> GLGDLIEGVVEGVTRNALTPLTPANNLPDTQSSGPAHSKETPALTAVETGATNPLVPSDTVQTRHVIQKRTRSESTVESFFARGACVAIIEVDNDAPTKRASKLFSIWKITYKDTVQLRRKLEFFTYSRFDMELTFVVTSNYTDANNGHALNQVYQIMYIPPGAPIPGKWNDYTWQTSSNPSLFYTYGAPPARISVPYVGIANAYSHFYDGFAKVPLAGQASTEGDSLYGAASLNDFGSLAVRVVNDHNPTKLTSKIRVYMKPKHVRVWCPRPPRAVPYYGPGVDYKDGLAPLPEKGLTTY;> MGAQVSSQKVGAHENSNRAYGGSTINYTTINYYRDSASNAASKQDFAQDPSKFTEPVKDVLIKTAPTLNSPNIEACGYSDRVMQLTLGNSTITTQEAANSVVAYGRWPEYIKDSEANPVDQPTEPAVAACRFYTLDTVTWRKESRGWWWKLPDALKDMGLFGQNMFYHYLGRAGYTVHVQCNASKFHQGALGVFAVPEMCLAGDSTTHMFTKYENANPGEKGGEFKGSFTLDTNATNPARNFCPVDYLFGSGVLAGNAFVYPHQIINLRTNNCATLVLPYVNSLSIDSMTKHNNWGIAILPLAPLDFATESSTEIPITLTIAPMCCEFNGLRNITVPRTQ;> GLPVLNTPGSNQYLTADNYQSPCAIPEFDVTPPIDIPGEVRNMM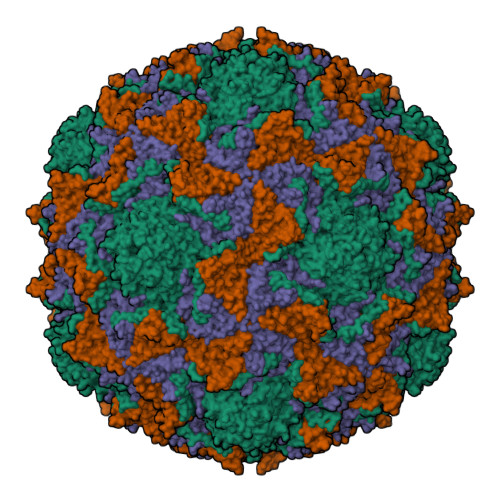ELAEIDTMIPLNLTNQRKNTMDMYRVELNDAAHSDTPILCLSLSPASDPRLAHTMLGEILNYYTHWAGSLKFTFLFCGSMMATGKLLVSYAPPGAEAPKSRKEAMLGTHVIWDIGLQSSCTMVVPWISNTTYRLTINDSFTEGGYISMFYQTRVVVPLSTPRKMDILGFVSACNDFSVRLLRDTTHISQEAMPQ> DPAGLLDLRQGMFAQLVAQNVLLIDGPLSWYSDPGLAGVSLTGGLSYKEDTKELVVAKAGVYYVFFQMELRRVVAGEGSGSVSLALHLMPLRSAAGAAALALTVDLPPASSEARNSAFGFQGRLLHLSAGQRLGVHLHTEARARHAWQLTQGATVL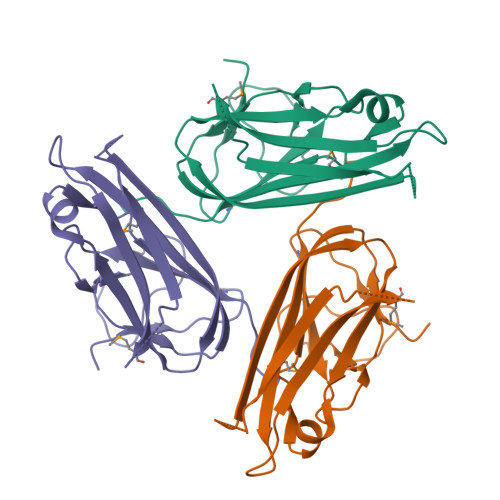GLFRVTPEIPA> WARTELLNVCMNAKHHKEKPGPEDKLHEQCRPWRKNACCSTNTS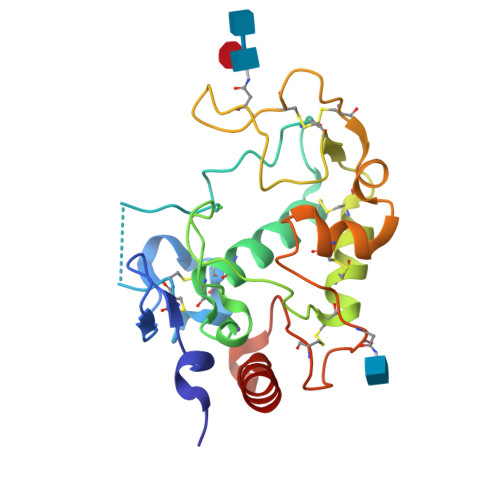QEAHKDVSYLYRFNWNHCGEMAPACKRHFIQDTCLYECSPNLGPWIQQVDQSWRKERVLNVPLCKEDCEQWWEDCRTSYTCKSNWHKGWNWTSGFNKCAVGAACQPFHFYFPTPTVLCNEIWTHSYKVSNYSRGSGRCIQMWFDPAQGNPNEEVARFYAAAMS> GPPDLGTDDDDKAMADIASDFPNNKETGEALLTPVDATASSHDGNGPDRLIDQDLTTRWSSAGDGEWAMLDYGSVQEFDAVQASFSKGNERQSKFDIQVSVDGETWTTVLENQLSSGKAIGLERFQFEPAVKARYVRYVGHGNTKNGWNSVTGLAAVNCSINACPASQIITSDVVAAEAVLIAEMKAAEKARKAARKDLRSGNFGVAAVYPCETSVKCDTRSALPVPTGLPATPVAGNAPSENFDMTHWYLSQPFDHDKNGKPDDVSEWNLANGYQHPEIFYTADDGGLVFKSYVKGVRTSKNTKYARTELREMMRRGDQSISTKGVNKNNWVFSSAPEADLEAAAGIDGVLEATLKIDHATTTGNANEVGRFIIGQIHDQNDEPIRLYYRKLPNQPTGAVYFAHESQDATKEDFYPLVGDMTAEVGEDGIALGEVFSYRIDVKGNTMTVTLMREGKDDVVQV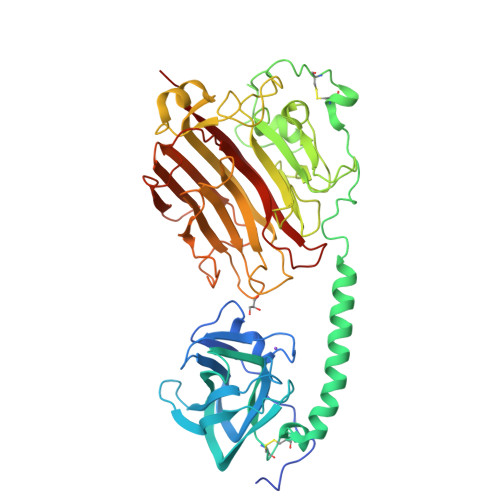VDMSNSGYDVGGKYMYFKAGVYNQNISGDLDDYSQATFYQLDVSHDQYKK>EIGTGFPFDPHYVEVLGSRMHYVDVGPRDGTPVLFLHGNPTSSYLWRNIIPHVAPSHRCIAPDLIGMGKSDKPDLDYRFDDHVRYLDAFIEALGLEEVVLVIHDWGSALGFHWAKRNPERVKGIAFMEFIRPIPTWDEW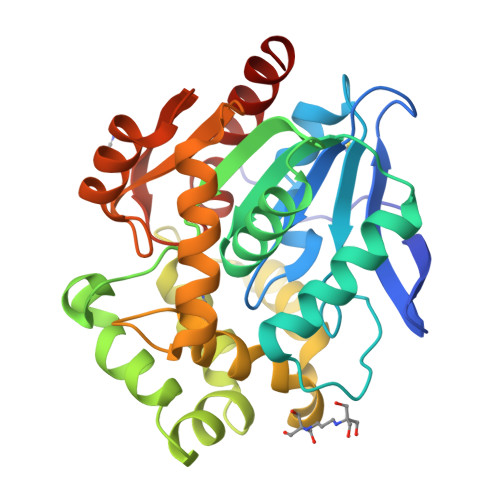PEFARELFQAFRTPDVGRELIIDQNAFIEGILPKFVVRPLTEVEMDHYREPFLKPVWREPLWRFPNELPIAGEPANIWALVEAYMNWLHQSPVPKLLFWGTPGVLIPPAEAARLAESLPNLKTVFIGPGLHYLQEDNPDLIGSEIARWLPAL[2x]>XFFGPQYQP[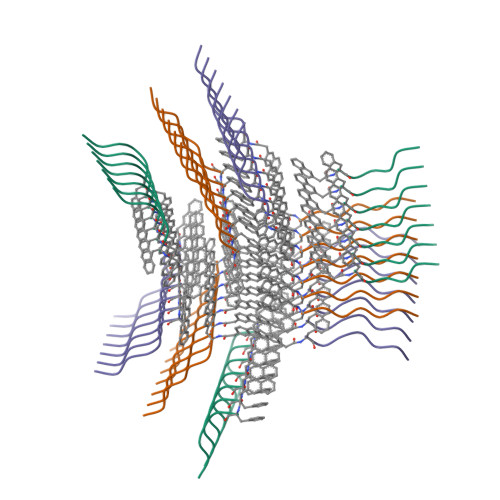3x]>GCUG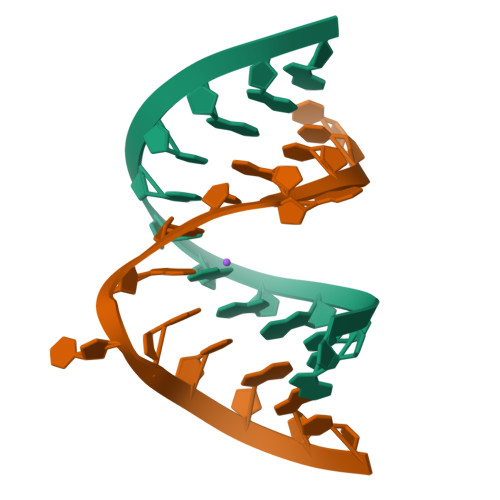GGCGCAGG[4x];>[4x]CCUGACGGUACAGC>GPGSELPQMVQQLNSPDQQELQSALRKLSQIASGGNEQIQAVIDAGALPALVQLLSSPNEQILQEALWALSNIASGGNEQIQAVIDAGALPALVQLLSSPNEQILQEALWALSNIASGGNEQIQAVIDAGALPALVQLLSSPNEQILQEALWALSNIASGGNEQIQAVIDAGALPALVQLLSSPNEQILQEALWALSNIASGGNEQIQAVIDAGALPALVQLLSSPNEQILQEALWALSNIASGGNEQKQAVKEAGA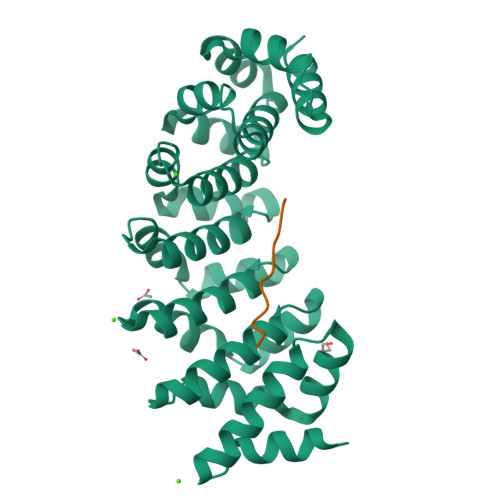LEKLEQLQSHENEKIQKEAQEALEKLQSH[3x];>KRKRKRKRKR[3x]>MIHLYDAKSFAKLRAAQYAAFHTDAPGSWFDHTSGVLESVEDGTPVLAIGVESGDAIVFDKNAQRIVAYKEKSVKAEDGSVSVVQVENGFMKQGHRGWLVDLTGELVGCSPVVAEFGGHRYASGMVIVTGKGNSGKTPLVHALGEALGGKDKYATVRFGEPLSGYNTDFNVFVDD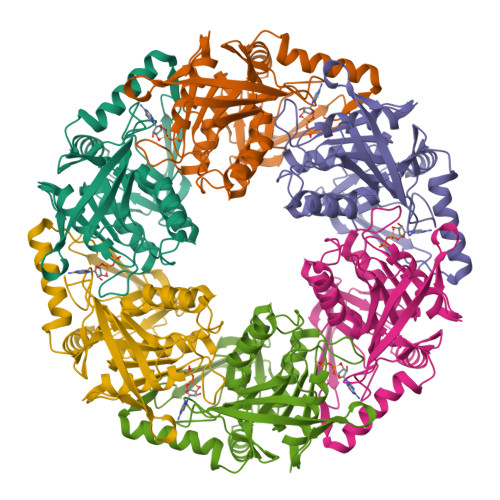IARAMLQHRVIVIDSLKNVIGAAGGNTTSGGISRGAFDLLSDIGAMAASRGCVVIASLNPTSNDDKIVELVKEASRANSTSLVISTDVDGEWQVLTRTGEGLQRLTHTLQTSYGEHSVLTIHTSKQSGGKQASGKAIQTVIKNDELESVLRRLTSN[3x]>GAMETITVPTPIKQIFSDDAFAETIKDNLKKKSVTDAVTQNELNSIDQIIANNSDIKSVQGIQYL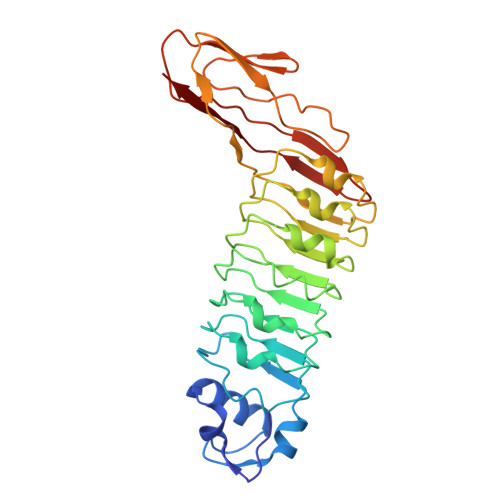PNVTKLFLNGNKLTDIKPLANLKNLGWLFLDENKVKDLSSLKDLKKLKSLSLEHNGISDINGLVHLPQLESLYLGNNKITDITVLSRLTKLDTLSLEDNQIRRIVPLARLTKLQNLYLSKNHISDLRALRGLKNLDVLELFSQEALNKPINHQSNLVVPNTVKNTDGSLVTPEIISDDGDYEKPNVKWHLPEFTNEVSFIFYQPVTIGKAKARFHGRVTQPLKE[2x]>[6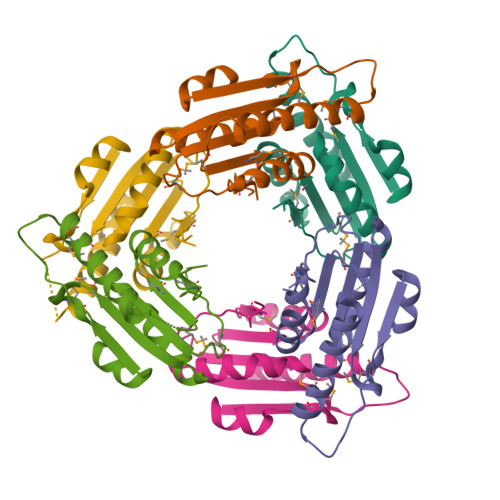x]MKEGDSLLNVAGPLGTPVPMEKFGKILAIGAYTGIVEVYPIAKAWQEIGNDVTTLHVTFEPMVILKEELEKAVTRHIVEPVPLNPNQDFLANMKNVSQRLKEKVRELLESEDWDLVFMVGPVGDQKQVFEVVKEYGVPMKVDLHPIMVDGLEHHHHHH> AAPFNGTMMQYFEWYLPDDGTLWTKVANEANNLSSLGITALWLPPAYKGTSRSDVGYG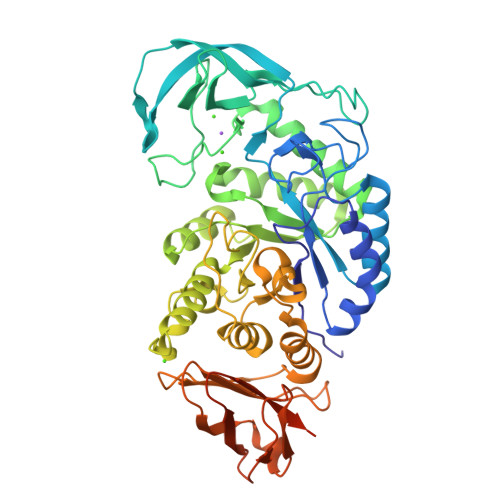VYDLYDLGEFNQKGAVRTKYGTKAQYLQAIQAAHAAGMQVYADVVFDHKGGADGTEWVDAVEVNPSDRNQEISGTYQIQAWTKFDFPGRGNTYSSFKWRWYHFDGVDWDESRKLSRIYKFRGIGKAWDWEVDTENGNYDYLMYADLDMDHPEVVTELKSWGKWYVNTTNIDGFRLDAVKHIKFSFFPDWLSYVRSQTGKPLFTVGEYWSYDINKLHNYIMKTNGTMSLFDAPLHNKFYTASKSGGTFDMRTLMTNTLMKDQPTLAVTFVDNHDTEPGQALQSWVDPWFKPLAYAFILTRQEGYPCVFYGDYYGIPQYNIPSLKSKIDPLLIARRDYAYGTQHDYLDHSDIIGWTREGVTEKPGSGLAALITDGPGGSKWMYVGKQHAGKVFYDLTGNRSDTVTINSDGWGEFKVNGGSVSVWVPRKTTVSTIAWSITTRPWTDEFVRWTEPRLVAWP>[2x]MTMASVPASRYLTDMTLEEMSRDWSMLIPKQKVAGPLCIRM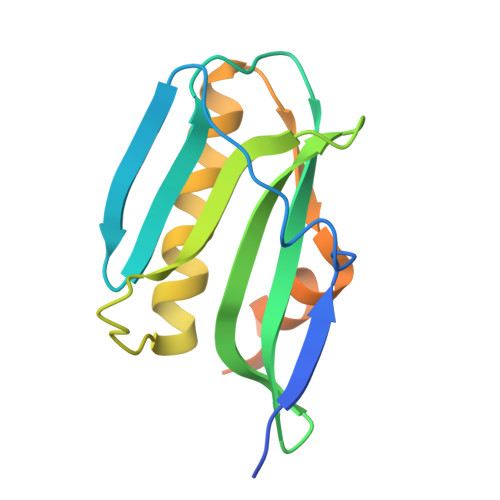DQAIMDKNIILKANFSVIFDRLETLILLRAFTEEGAIVGEISPLPSLPGHTAEDVKNAVGVLIGGLEANDNTVRVSETLQRFAWRSSNENGRPPLTPKQKREMAGTIRSEV>MARVKHFELLTDEGKTFTHVDLYGKYTILFFFPKAGTSGSTREAVEFSRENFEKAQVVGISRDSVEALKRFKEKNDLKVTLLSDPEGILHEFFNVLENGKTVRSTFLIDRWGFVRKEWRRVKVEGHVQEVKEALDRLIEEDLSLNKHIEWRRARRALKKDRVPREELELLIKAAHLAPSCMNNQPWRFVVVDEEELLKKIHEALPGGNYWMKNAPALIAVHSKKDFDCALPDNRDYFLFDTGLAVGNLLVQATQMGLVAHPVAGYDPVKVKEILKIPEDHVLITLIAVGYLGDESELSEKHREL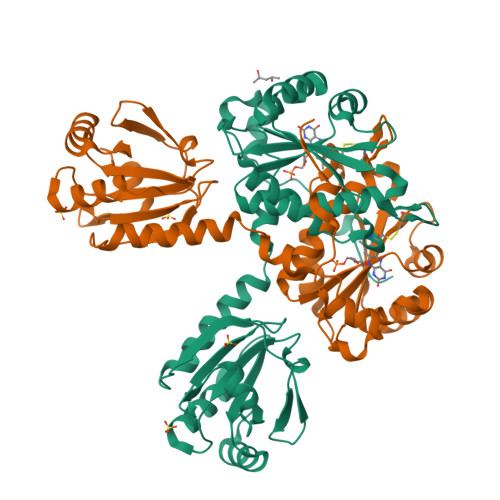ERSERVRKELSEIVRWNL[2x]> GSHMASMKKKGSVVIVGRINLSGDTAYAQQTRGEEGCQETSQTGRDKNQVEGEVQIVSTATQTFLATSINGVLWTVYHGAGTRTIASPKGPVTQMYTNVDKDLVGWQAPQGSRSLTPCTCG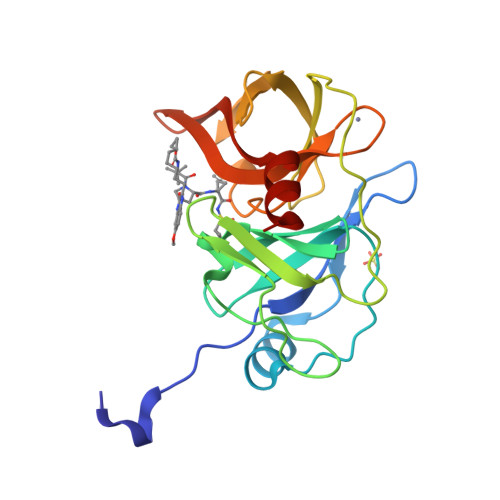SSDLYLVTRHADVIPVRRRGDSRGSLLSPRPISYLKGSAGGPLLCPAGHAVGIFRTAVSTRGVAKAVDFIPVESLETTMRSP> MNYSQIERMARKGVAFFTDPSRPMNLIKQGEYGYDENGFEIPPME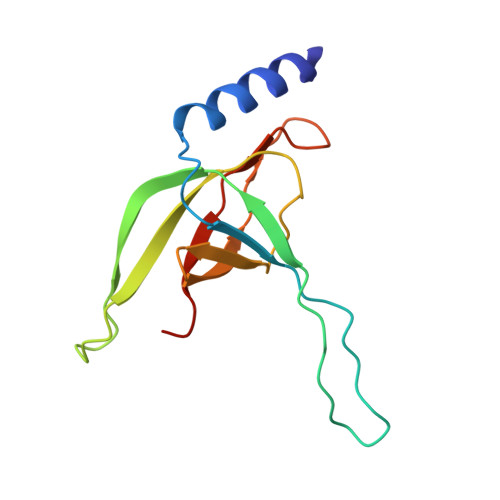QVIPISGATRRPNAREIDGETIRASDILGIFNNDHEINEGDYIEIDGIRHVVVDARPVQASLEPVAYRPVLRRVSVGG> MHHHHHHMLSHPPIPITDMAEHMERLKANDSLKLSQEYESIDPGQQFTWEHSNLEANKPKNRYANVIAYDHSRVILQPLEGIMGSDYINANYVDGYRRQNAYIATQGPLPETFGDFWRMVWEQRSATVVMMTRLEEKSRIKCDQYWPNRGTETYGFIQVTLLDTMELATFCVRTFSLHKNGSSEKREVRHFQFTAWPDHGVPEYPTPFLAFLRRVKTCNPPDAGPIVVHCSAGVGRTGCFIVIDAMLERIKTEKTVDVYGHVTLMRSQRNYMVQTEDQYGFIHEALLEAVGCGNTEVPARSLYTYIQKLAQVEPGEHVTGMELEFKRLASSKAHTSRFITASLPCNKFKNRLVNILPYESSRVCLQPIRGVEGSDYINASFIDGYRQQKAYIATQGPLAETTEDFWRALWENNSTIVVMLTKLREMGREKCHQYWPAERSARYQYFVVDPMAEYNMPQYILREFKVTDARDGQSRTVRQFQFTDWPEQGAPKSGEGFIDFIGQVHKTKEQFGQDGPISVHCSAGVGRTGVFITLSIVLERMRYEGVVDIFQTVKVLRTQRPAMVQTEDEYQFCFQAALE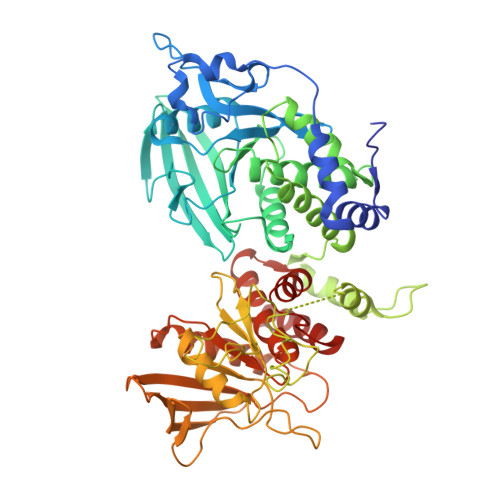YLGS~{tert}-butyl (2~{S})-2-[(1,3-dihydropyrrolo[3,4-c]pyridin-2-ylcarbonylamino)methyl]-6-azaspiro[2.5]octane-6-carboxylate 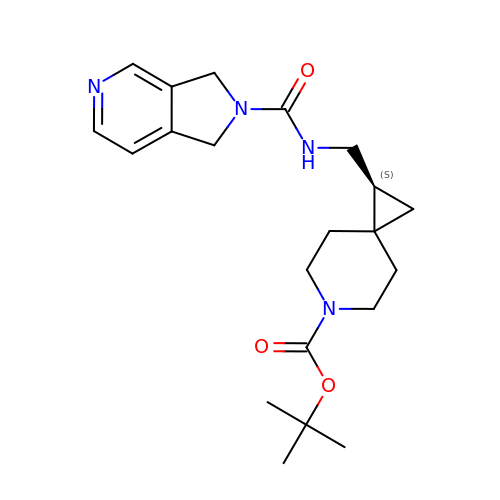| C21 H30 N4 O3 | DLHHFYXNVIMXSY-QGZVFWFLSA-N>[4x]SKKEILLDFIEKNNGIVTNKDCKALGIPTIYLTRLEKEGIIFRVEKGIFLTQNGDYDEYYFFQYRFPKAIFSYISALYLQQFTDEIPQYFDVTVPRGYRFNTPPANLNIHFVSKEYSELGMTTVPTPMGNNVRVYDFERIICDFVIHREKIDSELFVKTLQSYGNYPKKNLAKLYEYATKMNTLEKVKQTLEVLI

A recently characterized Abi system, AbiE from Streptococcus agalactiae V/R 2603, has been shown to act as a type IV TA system. AbiE encodes a DUF1814-family toxin (AbiEii), and a COG5340-family antitoxin (AbiEi). The antitoxin AbiEi from S. agalactiae has been biochemically characterized and functions as both an antitoxin and a transcriptional repressor. AbiEi contains an N-terminal winged helix-turn-helix DNA-binding domain and a C-terminal antitoxin domain, connected by a short linker.

To begin, we solved a 1.83 Å structure of AbiEi by X-ray crystallography. There were four copies of AbiEi in the asymmetric unit, forming minor crystal contacts that are not predicted to be biologically relevant, and each copy contains minor variations in domain orientation, indicating some flexibility. Together with previous size exclusion chromatography data, we concluded that AbiEi is a 23 kDa monomer in solution. The N-terminal domain contains three α-helices, followed by three beta-strands forming an antiparallel sheet. The C-terminal domain begins with a single α-helix that is separated from a six-helix bundle by a row of four β-strands, which themselves pair into parallel and antiparallel β-sheets. One face of AbiEi is positively charged, and the reverse face is negatively charged. The positive side corresponds with the site of positively charged sidechains distributed throughout the N-terminal and C-terminal domains, which have previously been shown to be vital for DNA-binding and autoregulation through mutagenesis studies. When AbiEi and Rv2827c are aligned via the N-terminal winged helix-turn-helix domain, the respective C-terminal domains differ in position relative to the N-terminal domains by ∼65°. In the AbiEi monomer, 16 identified residues were clustered at the C-terminus, forming a putative site for interaction. Overall, despite differing captured poses and discrepancy in size, AbiEi and Rv2827c are markedly similar in domain structure, fold and surface charge and are therefore structural homologs.> MSQSVTVIGLGPMGQAMAAAYLDRGYEVTLWNRTASRADALVARGAKLAATPEQALSANELVILSLIDYDAMYGVLEGAEEAVAGRVLVNLSSDTPEKARAAARRVAELGGTHLTGGVLSPPPGIGSPDMSTFYSGPRAAYDQHRAALEVITGKTDYRGEDPGLAALMYQLNMVVFWPAMLSYWQAVALADAHGLTAADIAPYVSENFAGMGQFIDFY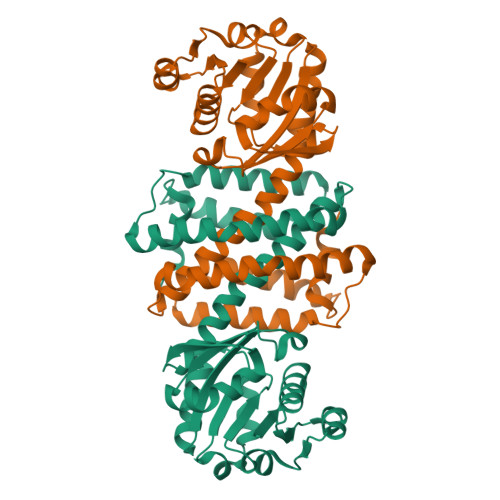AARIDAGNHAGDVDRLSMGVASMEHVVHTNADSGVDTAFPRAVLDAFHRGADAGFGADSFSSVIKLMKKQP> MGSSHHHHHHHSSGRENLYFQGHMEGVRWAFSCGTWLPSRAEWLLAVRSIQPEEKERIGQFVFARDAKAAMAGRLMIRKLVAEKLNIPWNHIRLQRTAKGKPVLAKDSSNPYPNFNFNISHQGDYAVLAAEPELQVGIDIMKTSFPGRGSIPEFFHIMKRKFTNKEWETIRSFKDEWTQLDMFYRNWALKESFIKAIGVGLGFELQRLEFDLSPLNLD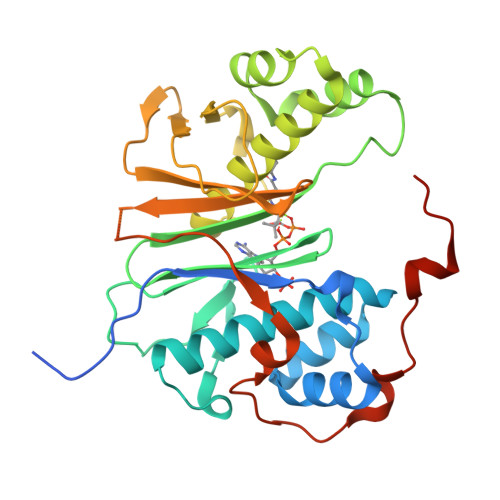IGQVYKETRLFLDGEEEKEWAFEESKIDEHHFVAVALRKPDGSRHQDVPSQDDSKPTQRQFTILNFNDLMSSAVPMTPEDPSFWDCFCFTEEIPIRNGTKSLESG> GPLGSMTQNNAPESVAAEGTVAGQQTDTTKPEPSSQPAPEPPSQVTTDFPPNNKPNDVPATEPASSSPRPTEPPAPPPPKPTIALSPLDIATLTFPDGTRGTFPAPPQTSAQSVSTPSIASGHVTPQRDTDTASITSVAGTLRGVTGTAGDLASLLAGDGLGRKSKAWRVLRAQQQACGEGSGEEGEITEIEGLGLGEGMEGFERELDNIPDTLPDDERLALWKGKLKHYLILSSAGKPIWSRHGDLSLVNSTMGVVQTIISFYEGARNPLLGFTAGKVRFVILIKGPLYFVAISRLRESDAQLRAQLEALYMQILSTLTLPILTNIFAHRPSTDLRGPLQGTESLLASLADSFTKGSPSTLLSALECLRLRKSQRQAITNIFLKSRCEELLYGLLVAGGKLVSVIRPRKHSLHPSDLQLIFNMLFESGGIKGNGGENWIPLCLPAFNNTGYLYMYVSFLDDKAPDDQNQPPESSNLDASNKNSSNTPDDDLTALILISPSREAFYALQSMRTRLVSQLLSTGYLSLIRSTALSGRPSITSILPKTPLLHFLYKSRPNVQWCMSSLSSLTPPGATATETLLARRKLMSVYEELHAALHARHAHLRVVYSTADEKEGEGLACLGWSTPAFEVYCVAPGCVGRAGMAREVNRVVQWARREEERLFILGGGVF;> SMTTPVSPSPSGIIPAQLGFLAIYNPALGTTDETLEDQIVYYATASTLSQARRRHRRPRRRDRQRAQSVVKDSRPNAAGATGDSEAVAEDKDPVSKEERHERLRQIGLAQGMVEFAKSFSDGEPVDTIDTEKARVILVEVEEGWWILASIDLTRLPLPQIKTPTSSSAPPP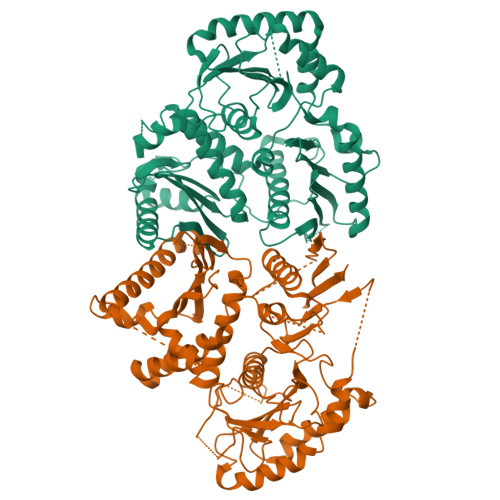APNLNPLPPEPAYEYSSREVKPPSLLRADLLRAYDLFLLHHGSSLSSLLASQGRAQLVASLTRFWDHFLATWNVLLHGNPACDVFGGIKLAASGELGIGVGEEERGSGEREVLEGLVERVEGLVDVVVGRYGGPPSEKGPEEEQWLGLGGEVGEEDGAVFLGVGALDRKSLRGVVQWMEEVYVWGENAFGKPRRDLSTGHFLLGLSECSEEELTSSQANPKAIFVELKPSYQHPSRKIPPEDPQPLGKVGPELPRDHTARLRPVIYVSQPFIYILLFSEITPSPSTWPTLAESLHAQLSPLQKPLLHSTSYRPERPVVETTSSSGTTTQHQIFDLVYDTETLTLQSTIPNIPDPFPYSATTPTGHSTGQQHHQQSIWTRVEALQTHAQILAILSSGRAIPTDPSSFTHLPWEEGERTCKTARGWWIVWTRVVEHSPPDAVSLHHARDDDDNDDDASCSVLGHLRSVSSSHAAGSTSSSSGSGFGLGAIPGLGGLGGWAADGATRLAQGIGIDTRRYVEGLLTSLGR>[2x]MQEAARRASLRKEHTPTNEKFGDLSKQDSLGERASSKLTLDDELYDILYAFGETDAFINKGDKQRETDEDGNPLTRQALLERIRQKKEVIGKLRCQAWSMTRKRRTLKLAQKYLEQHESKVSRSHLYMEEMRKRARLMKRSFSNFKTYLIPWESKIKRIESHFGSVVSSYFTFLRWIVFVNIMITLIALVFVVLPETLADSVANEGRFNRTKTRKQIPANERVHADELAVVWHYDGYLRYSPLFYGYYSDDPFLGNKIKYALPLAYFMVTLTIFAYSFFAILRKMAANARMSKLSGSKAEQYIFNWKLFTGWDYTIGNSETASNTVMAVVIKLRESIADIKKDAHGKFRLLQFSLRVFANIIICAMLGFSIYCIIFAVQKSQVQDDGNLFTKNQVPSVVSTITHVFPMIFDLIGKMENYHPRTALRAHLGRVLILYTVNYITLIFALFEKMTALRDRVNSTSTSSSHRTKRQQGGWNPNMQRPPPYASRAEVRQMSDFLAANTRR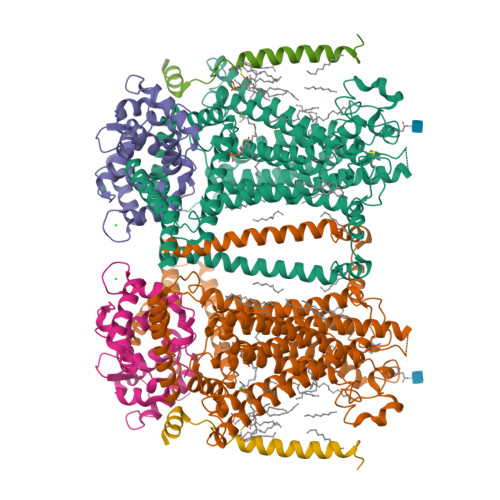FQTVSQRTTRSVTTPFTVAPQFGPFNVNNPNAVFHNGTHSTSFESQILGPKALPIFTPPPRKYPGFTPGNVGQQFGGPDFPRNQVYTKSTPLPRVRTKPPWVYTTTHPPLVQNRAMTTTMSKSAKKGNSKNLDDDILLSNETIQMSEAALRRNHDGHNNDICWETIIGQEIVKLVTMDLIFTILSILVIDLFRGLWIKYCSSWWCWDIETTFPEYGEFKVAENVLHIINNQGMIWLGLFFAPLLPAINNIKLIILMYIRGWAVMTCNVPAREIFRASRSSNFYLGILLIWLLLCTLPVGFVIASMSPSRSCGPFARYQHFYTVVTREIEKRVDQTVLSYIRHIASPGVVIPIILFLILIIYFLFSLVRGLREANTDLQAQLVHERTEEKKKIFELAGGKKNKFEKDRDKKRSNDYIPLIEQRRREPWRQYHEMEADHALASDSSEESDINEDEDDERQPLTAYPLRAIETPPETLQVTAFHPSLGSLIENREMEDEESASGDQLPMIHKSVSFQGPSHMQMRQSISTESCSQISRSAIQVATPEEIRALLRPYLEAKYGIPYQHGIKSFPIDVHTPPNNTPSRRSSKYNSFVSLYEHTRDDHKNFVASTIKETDEDPGKSDKKQTSSKDVAPDFMPWPSADEARALREKMKSKTPLMLTKTTVEEKPKGGKSSESEFRPPVPIHRKYNIQTTEEENEEEETDSAPESSKKRFRISVSPTKTIAPASASRAQHKIVSQASSSSSIPHGRQPDPNKKASLVLPPLRAPRVQFDEDDSPRQID;>MGNNASSLSELNLFSKGGVFTREQLDEYQDCTFFTRKDIIRLYKRFYALNPHKVPTNMQGNRPAITTLTFEEVEKMPELKENPFKRRICEVFSEDGRGNLSFDDFLDMFSVFSEMAPLQLKLKYAFRIYDYDGDELLGHDDLSKMIRSLTRDELSDVEVEFIIERIIEEADLDGDSSINFAEFEHVVSRSPDFIRTFHIRI[2x];>MPSGNEEINHLSALDQFVAPGLRLWMLIALVGGVLLIMIVIVCCFMRIRIPRTKRQIDLIAAKRKLRKSTKNSAEANAHNDERAQAIVMNSMPSGGGGGAPSTSSSRHTGSRIQSQV[2x]>MNNMNVIIADDHPIVLFGIRKSLEQIEWVNVVGEFEDSTALINNLPKLDAHVLITDLSMPGDKYGDGITLIKYIKRHFPSLSIIVLTMNNNPAILSAVLDLDIEGIVLKQGAPTDLPKALAALQKGKKFTPESVSRLLEKISAGGYGDKRLSPKESEVLRLFAEGFLVTEIAKKLNRSIKTISSQKKSAMMKLGVENDIALLNYLSSVT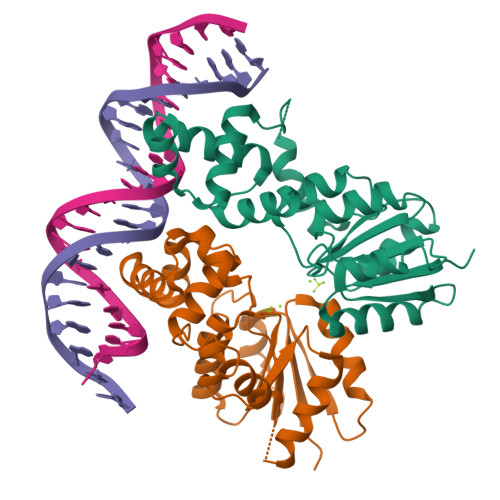LSPTDKE[2x]N-[(phenylcarbonyl)carbamoyl]-beta-D-glucopyranosylamine | C14 H18 N2 O7 | 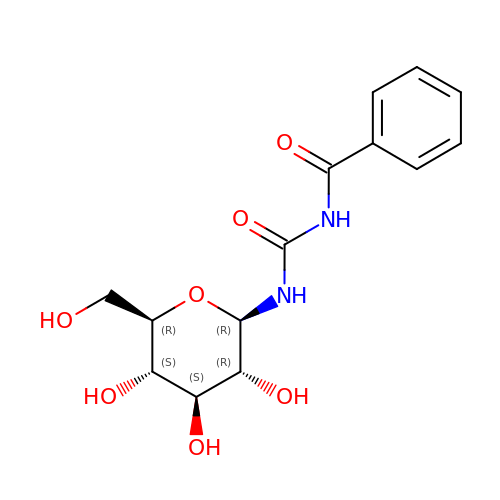JSBCZGSPFATCOV-BZNQNGANSA-N2-amino-5-fluorobenzoic acid | C7 H6 F N O2 | 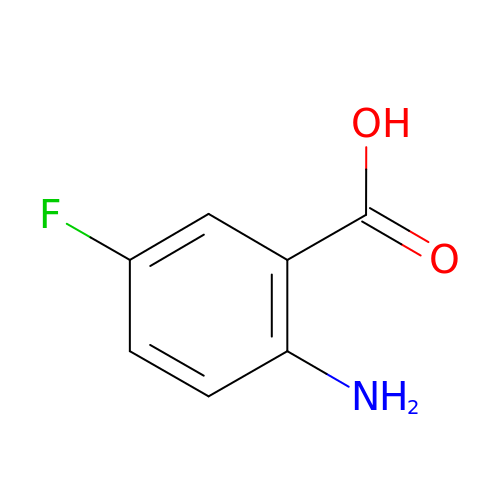FPQMGQZTBWIHDN-UHFFFAOYSA-N Drosophila melanogaster α-amylase, DMA, which belongs to the glycoside hydrolase family 13, sub family 15, has been studied from an evolutionary, biochemical, and structural point of view. Indeed, plant produced inhibitors are an important element of the plant defense response to insect predation against feeding. α-Amylases (α-1,4-glucan-4-glucanohydrolase, EC 3.2.1.1) belong to the glycoside hydrolase family 13 (GH13) as classified in the CAZy database, and catalyze the hydrolysis of starch and related α-1,4-linked glycosyl polysaccharides. As reported for other α-amylases from mammals, insect, plants, fungi, archaea and bacterial α-amylases, the enzyme consists of three distinct domains, A (residues 1 to 97 and 160 to 379), B (residues 98 to 159) and C (residues 380 to 476). In DMA, the nucleophile is Asp186, the general acid/base catalyst Glu223 and the transition state stabilizer is Asp288.

Crystals of DMA belong to the monoclinic space group P21, and two molecules of DMA are present in the asymmetric unit. Structure solution was performed by molecular replacement, using the known three-dimensional structure of TMA with which DMA presents 63% sequence identity as a search model. Domain A, which hosts the active site of the enzyme, displays a (β/α)8-barrel fold. Domain B is characterized by its high variability in α-amylases depending on the origin, and as in other reported structures it is flanked by β3 and α3, and participates in binding a conserved calcium ion (here substituted with strontium due to crystallization conditions) at the interface with domain A. This metal ion contributes to the enzyme’s structural integrity. Domain C in the C-terminal part of the protein is composed of an eight-stranded anti-parallel β-sheet. Apart from the above mentioned conserved structural calcium ion, a chloride ion is located in the vicinity of the active site and a second non-conserved and highly solvated metal ion was identified in the electron density. In DMA the conserved calcium ion is coordinated by three water molecules, and residues from domain A (Asn98 OD1, Arg147 O, Asp156 OD1 and Asp156 OD2) and from domain B His190 O. Arg147 belongs to a well conserved motif and is present in more than 300 known animal Amy sequences, but not in Caenorhabditis elegans (Lys), nor in the paralog Amyrel present in true flies (Muscomorpha), which has a glutamine instead. In the DMA three-dimensional structure a chloride anion is present and is coordinated by Arg184 and Asn286 and Arg325. The non-conserved metal ion which has been identified in the electron density is highly solvated, being ligated to six water molecules, and performs only one direct coordination bond to the enzyme Gln263 which is weakly conserved, even within Drosphila. Apart from this direct coordination, the only contact this ion has with DMA is via a water molecule to Asp391, a residue which is conserved in all Drosophila except D. pseudoobscura.

>[2x]MFLAKSIVCLALLAVANAQFDTNYASGRSGMVHLFEWKWDDIAAECENFLGPNGYAGVQVSPVNENAVKDSRPWWERYQPISYKLETRSGNEEQFASMVKRCNAVGVRTYVDVVFNHMAADGGTYGTGGSTASPSSKSYPGVPYSSLDFNPTCAISNYNDANEVRNCELVGLRDLNQGNSYVQDKVVEFLDHLIDLGVAGFRVDAAKHMWPADLAVIYGRLKNLNTDHGFASGSKAYIVQEVIDMGGEAISKSEYTGLGAITEFRHSDSIGKVFRGKDQLQYLTNWGTAWGFAASDRSLVFVDNHDNQRGHGAGGADVLTYKVPKQYKMASAFMLAHPFGTPRVMSSFSFTDTDQGPPTTDGHNIASPIFNSDNSCSGGWVCEHRWRQIYNMVAFRNAVGSDEIQNWWDNGSNQISFSRGSRGFVAFNNDNYDLNSSLQTGLPAGTYCDVISGSKSGSSCTGKTVTVGSDGRASINIGSSEDDGVLAIHVNAKL O. alaskensis employs a tripartite ATP-independent periplasmic (TRAP) transporter (OaIsePQM) to import isethionate, which relies on the substrate-binding protein (OaIseP) to scavenge isethionate and deliver it to the membrane transporter component (OaIseQM) for import into the cell. Like the ATP-binding cassette importers, TRAP transporters utilise a high-affinity substrate-binding protein (P-subunit) that binds the organic acid and delivers it to the membrane-spanning transporter subunits (Q and M) for uptake. The structure of TRAP substrate-binding proteins comprises two globular lobe-like domains connected by a variable hinge region, which is formed by two β-strands and a unique extended α-helix. Substrates bind within the cleft between the two domains, which close around the bound substrate via a hinge-bending conformational change often described as a ‘Venus flytrap’ mechanism.

Of these three datasets, only the 1.48 Å dataset was truly ligand-free, whereas the other two datasets had sulfonate-containing buffering compounds [4-(2-hydroxyethyl)-1-piperazineethanesulfonic acid (HEPES) and 2-(N-morpholino)ethanesulfonic acid (MES)] in the substrate-binding site arising from the crystallisation condition (see crystallisation and structure determination methods). We had suspected OaIseP had tightly bound a non-cognate ligand present during expression in E. coli, a phenomenon that is not uncommon for TRAP substrate-binding proteins as documented by Vetting et al.. Upon further refinement, we were able to confidently model HEPES and MES buffer constituents from the crystallisation conditions into the densities (difference maps shown in Supplementary Figure S5) and refined the structures to an Rfree of 0.229 (1.89 Å resolution) and 0.241 (1.65 Å resolution) respectively. In both HEPES- and MES-bound structures, the sulfonate groups form a salt bridge to Arg177 and hydrogen bonding the side chain nitrogen of Asn217. In the HEPES-bound structure, Arg156 is tilted slightly further from the sulfonate group, only granting a single nitrogen atom of the guanidyl group to form hydrogen bonds with the HEPES sulfonate, whereas Arg156 is turned slightly closer to the MES sulfonate allowing the respective salt bridge to form. The smaller MES utilises a bridging water molecule hydrogen bond Ala40 to the morpholine ring oxygen. In contrast, it is interesting that the slightly smaller MES does not induce partial closure, considering the water molecule bridging the hydrogen bond with Ala40 could be removed and a direct hydrogen bond could be formed instead. The melting temperature of OaIseP (TmD) in the presence of MES (5 mM, 58.5 ± 0.3°C) and HEPES (5 mM, 57.0 ± 0.6°C) is not significantly different to that of ligand-free OaIseP (ΔTmD of 0.6°C and −0.9°C, respectively). This suggests that these molecules bind weakly, or that it is the full closure of the protein around the ligand that induces thermal stability.

> MKHLLKAGALVALACIVTLTAGAQAHAAKRINIRLAHPMAPGNNVTVGYEKFKELVAEKSNGRVRIQLFGNCMLGSDRVTMEAAQRGTLEMASSSSPNMANFSKQWMVFDLPYITSPEHQQKLYKAIDDGELGKKLDEIAASIGLKPIMYSEYGYRNFVTTKKPIKTADDLKNLKVRTTDSPIEVAVAAALGMAPTPISWGETYTALQQGTVDGEGNTFSLLNDAKHTEVLKYAIDSAHNYSMHLLMMNKAYYDSLPANVQQILTEAGREALTYQRSITSELEKKAEDAFIEQGITVTRLSPEERAKLVERTRPVWDKFKDDIPAELIKLVQETQQ> AYRPSETLCGGELVDTLQFVCGDRG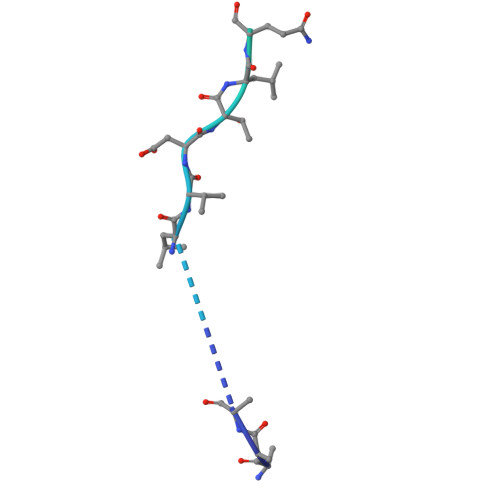FYFSRPASRVSRRSRGIVEECCFRSCDLALLETYCATPAKSE5-(4-{3-[(2,4-diamino-6-ethylpyrimidin-5-yl)oxy]propoxy}phenyl)-6-ethylpyrimidine-2,4-diamine | C21 H28 N8 O2 | 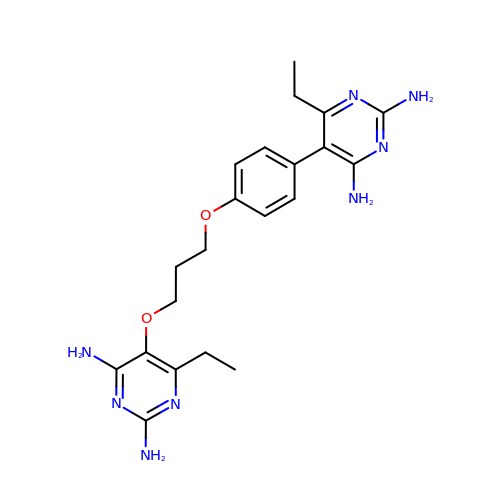VSAKYGGFYNIPDW-UHFFFAOYSA-N> KRIVACDDPDFLTS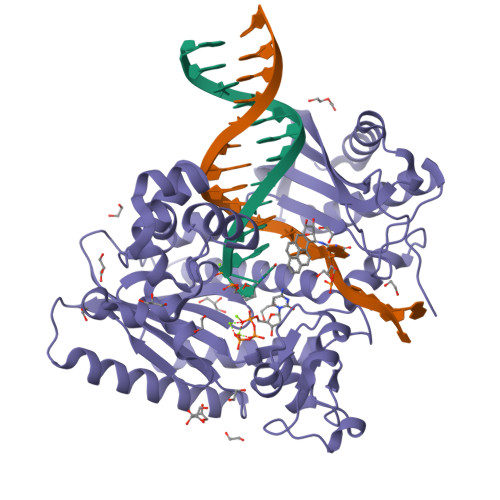YFAHSRLHHLSAWKANLKDKFLNENIHKYTKITDKDTYIIFHIDFDCFFATVAYLCRSSSFSACDFKRDPIVVCHGTKNSDIASCNYVARSYGIKNGMWVSQAEKMLPNGIKLISLPYTFEQFQLKSEAFYSTLKRLNIFNLILPISIDEAVCVRIIPDNIHNTNTLNARLCEEIRQEIFQGTNGCTVSIGCSDSLVLARLALKMAKPNGYNITFKSNLSEEFWSSFKLDDLPGVGHSTLSRLESTFDSPHSLNDLRKRYTLDALKASVGSKLGMKIHLALQGQDDEESLKILYDPKEVLQRKSLSIDINWGIRFKNITQVDLFIERGCQYLLEKLNEINKTTSQITLKLMRRCKDAPIEPPKYMGMGRCDSFSRSSRLGIPTNEFGIIATEMKSLYRTLGCPPMELRGLALQFNKLVDV> MWGNLWTEASYQLNFNIGFSSLRSDVLIHLAQWQYWWWFWFALIWSFYYFIILKVARFRVLKMRPKISTSYRPHGKWGDFLACIIPLIWCINILTNSNLILRLIEWQNESSLFTVRVRARQWYWIYKFELKNFTDILSTPKNIGNNRWQINTFGELQTADDYLHVLQLRSQNKWVKNYWNRSLQETGKTNKAHVISPQEQLRLSLINQYKSLNLSSSIKHNAPFINRDLYVFDDLFSYNLGDITTKKSLFNDKNSFLTSYSYLNNNSWNNNEFDLIDNLPFTTLFDNNDLFNNYKSFFQDSIFNSPKKQLSSDSKQL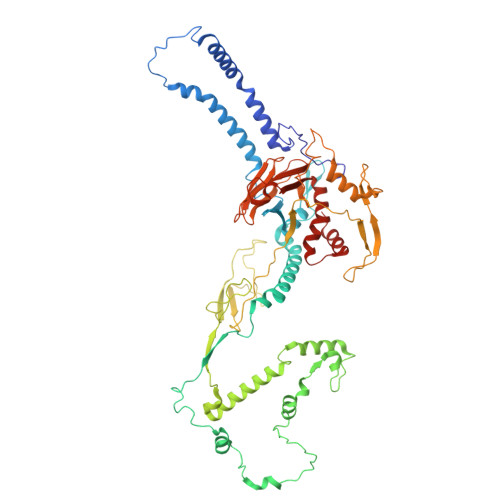FKHIIYRSIKNNIIQDYTKLVKHEDFDEYSRWIKRSPGEVLPLRIIKYPLGLETIHNNIFENTNNEGNVELFRLRFNSNSSKMQHKLVQDTIYLTLKQKRYNRKKVVAPQIKYYKDDNGNKTDLVKYTGKPYLSNDKLLKQSIYDQTTQYKLIKKNKKRGELIPVTLARRILRTKKTLVLPAHVNITLITNSYDIVHSWFIPGLGIKLDCVPGRSTHHTFFIDNVGFYYGQCAEICGRYHHHMPIRVCALPFEHFLLWWNTFGLPKMLNTVSRKRFETHYELRKYSW>MHGSNKLPGFATRAIHHGYDPQDHGGALVPPVYQTATFTFPTVEYGAACFAGEQAGHFYSRISNPTLNLLEARMASLEGGEAGLAL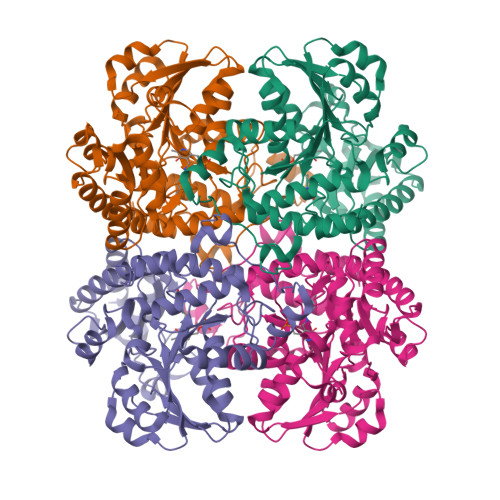ASGMGAITSTLWTLLRPGDEVLLGNTLYGCTFAFLHHGIGEFGVKLRHVDMADLQALEAAMTPATRVIYFESPANPNMHMADIAGVAKIARKHGATVVVDNTYCTPYLQRPLELGADLVVHSATKYLSGHGDITAGIVVGSQALVDRIRLQGLKDMTGAVLSPHDAALLMRGIKTLNLRMDRHCANAQVLAEFLARQPQVELIHYPGLASFPQYTLARQQMSQPGGMIAFELKGGIGAGRRFMNALQLFSRAVSLGDAESLASHPASMTHSSYTPEERAHYGISEGLVRLSVGLEDIDDLLADVQQALKASA[4x]> MTR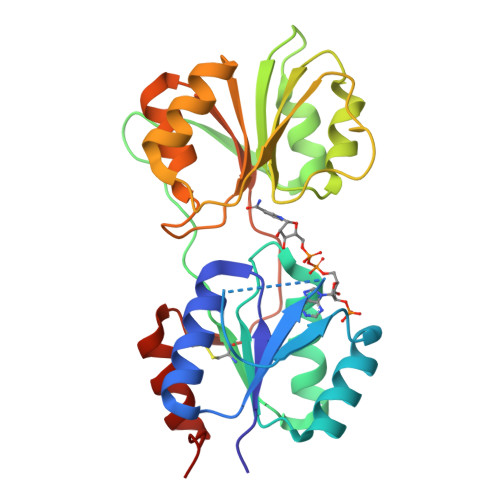LLVLGGTTEASRLAKTLADQGFEAVFSYAGRTGAPVAQPLPTRIGGFGGVAGLVDYLTREGVSHVIDATHPFAAQMSANAVAACAQTGVALCAFERAPWTAQAGDRWTHVPDLAAAVAALPQAPARVFLAIGKQHLRDFSAAPQHHYLLRLVDPPEGPLPLPDARAVIARGPFTVQGDTELLRSETITHVVAKNAGGAGAEAKLIAARSLGLPVILIDRPAVPARDICATLEGVMGWLADHGATPRGV> MEDLSSLTPGGSMGLQVNRGSQSSLEGAPATAPEPHSLGILHASYSVSHRVRPWWDITSCRQQWTRQILKDVSLYVESGQIMCILGSSGSGKTTLLDAMSGRLGRAGTFLGEVYVNGRALRREQFQDCFSYVLQSDTLLSSLTVRETLHYTALLAIRRGNPGSFQKKVEAVMAELSLSHVADRLIGNYSLGGISTGERRRVSIAAQLLQDPKVMLFDEPTTGLDCMTANQIVVLLVELARRNRIVVLTIHQPRSELFQLFDKIAILSFGELIFCGTPAEMLDFFNDCGYPCPEHSNPFDFYMDLTSVDTQSKEREIETSKRVQMIESAYKKSAICHKTLKNIERMKHLKTLPMVPFKTKDSPGVFSKLGVLLRRVTRNLVRNKLAVITRLLQNLIMGLFLLFFVLRVRSNVLKGAIQDRVGLLYQFVGATPYTGMLNAVNLFPVLRAVSDQESQDGLYQKWQMMLAYALHVLPFSVVATMIFSSVCYWTLGLHPEVARFGYFSAALLAPHLIGEFLTLVLLGIVQNPNIVNSVVALLSIAGVLVGSGFLRNIQEMPIPFKIISYFTFQKYCSEILVVNEFYGLNFTCGSSNVSVTTNP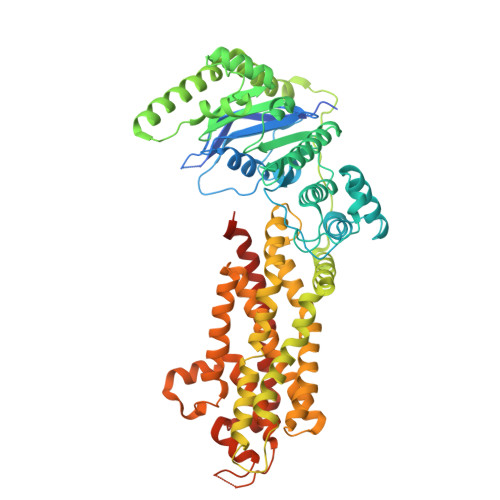MCAFTQGIQFIEKTCPGATSRFTMNFLILYSFIPALVILGIVVFKIRDHLISRGSHHHHHHGHHHHHH> GTERKLLERSRRLQEESKRLLDEMAEIMRRIKKLLKKAR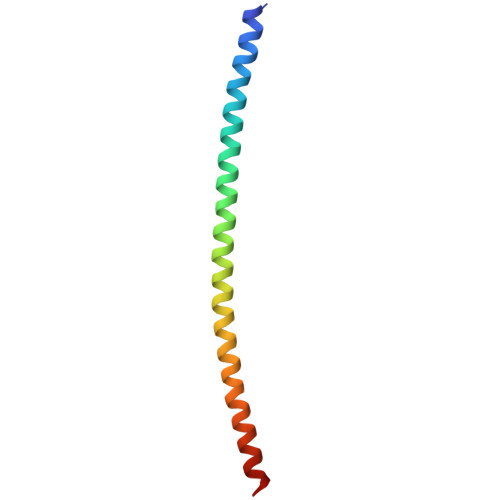GADEKVLDELRKIIERIRELLDRSRKIHERSEEIAYKEE> GAMSSSHHYSHPGGGGEQLAINELISDGSVVCAEALWDHVTMDDQELGFKAGDVIEVMDATNREWWWGRVADGEGWFPASFVRLRVNQDEPADDDAPLAGNSGAEDGGAEAQSSKDQMRTNVINEILSTERDYIKHLRDICEGYVRQCRKRADMFSEEQLRTIFGNIEDIYRCQKAFVKALEQRFNRERPHLSELGACFLEHQADFQIYSEYCNNHPNACVELSRLTKLSKYVYFFEACRLLQKM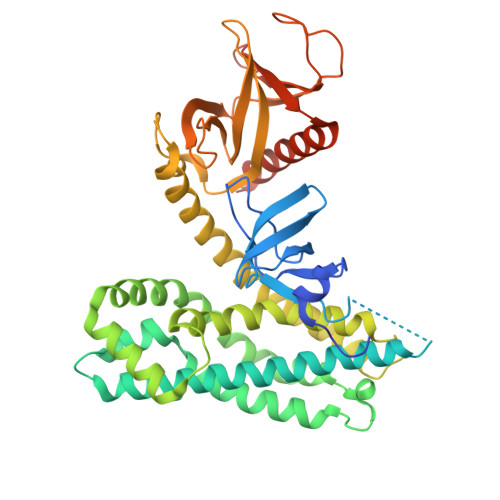IDISLDGFLLTPVQKICKYPLQLAELLKYTHPQHRDFKDVEAALHAMKNVAQLINERKRRLENIDKIAQWQSSIEDWEGEDLLVRSSELIYSGELTRVTQPQAKSQQRMFFLFDHQLIYCKKDLLRRDVLYYKGRLDMDGLEVVDLEDGKDRDLHVSIKNAFRLHRGATGDSHLLCTRKPEQKQRWLKAFAREREQVQLDQETGFSITELQRKQAMLNASK>GSARGMALYEEEQVERIGDIEERGKILVSLMYSTQQGGLIVGIIRCVHLAAMDANGYSDPFVKLWLKPDMGKKAKHKTQIKKKTLNPEFNEEFFYDIKHSDLAKKSLDISVWDYDIGKSNDYIGGCQLGISAKGERLKHWYECL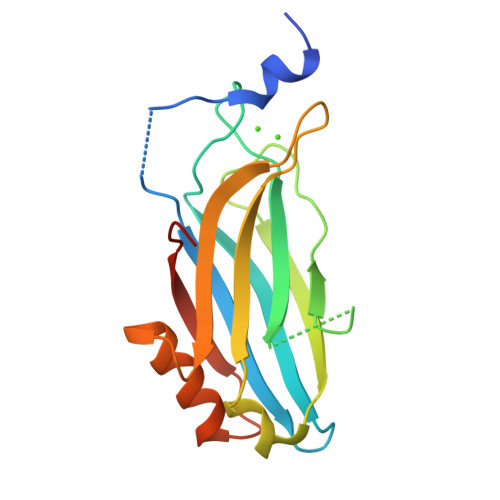KNKDKKIERWHQLQNENHVSSD[2x]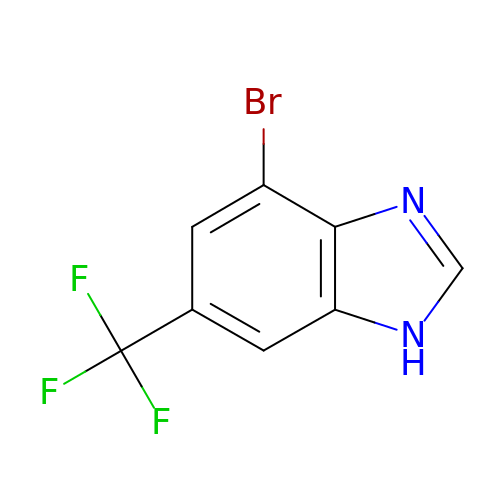4-bromanyl-6-(trifluoromethyl)-1~{H}-benzimidazole | C8 H4 Br F3 N2 | HYTQERQCUFICAX-UHFFFAOYSA-N> MDAELAEVRALQAEIAALRRACEDPPAPWEEKSR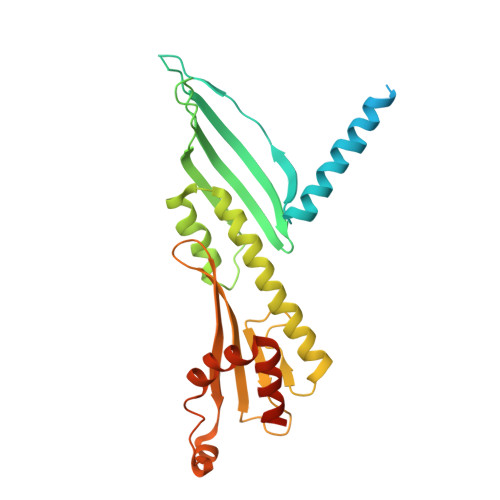VQKSFQAIHQFNLEGWKSSKDLKNQLGHLESELSFLSTLTGINIRNHSKQTEDLTSTEMTEKSIRKVLQRHRLSGNCHMVTFQLEFQILEIQNKERLSSAVTDLNIIMEPTECSELSEFVSRAEERKDLFMFFRSLHFFVEWFEYRKRTFKHLKEKYPDAVYLSEGPSSCSMGIRSASRPGFELVIVWRIQIDEDGKVFPKLDLLTKVPQRALELDKNRAIETAPLSFRTLVGLLGIEAALESLIKSLCAEENNENLYFQ> IRCNDKCYCEDGYARDVNGKCIPI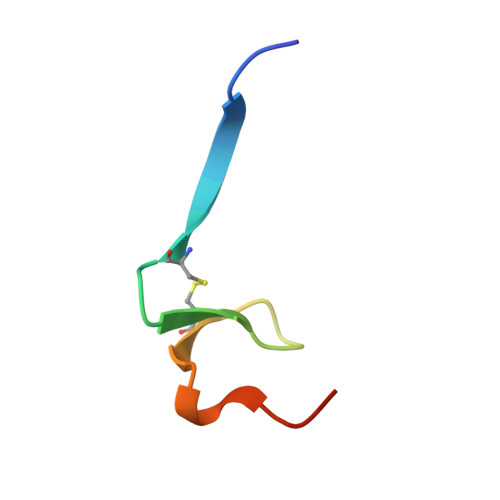KDCPKIRS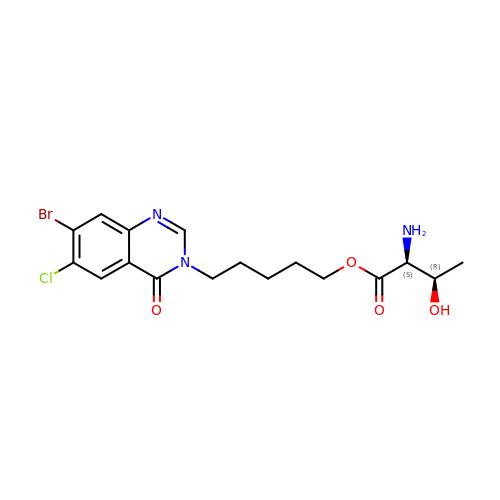5-(7-bromanyl-6-chloranyl-4-oxidanylidene-quinazolin-3-yl)pentyl (2~{S},3~{R})-2-azanyl-3-oxidanyl-butanoate | C17 H21 Br Cl N3 O4 | STFFHZKFSKKMRC-BMIGLBTASA-N>[2x]GSMAKIEKNAPTMEKKPELFNIMEVDGVPTLILSKEWWEKVCNFQAKPDDLILATYPKSGTTWMHEILDMILNDGDVEKCKRAQTLDRHAFLELKF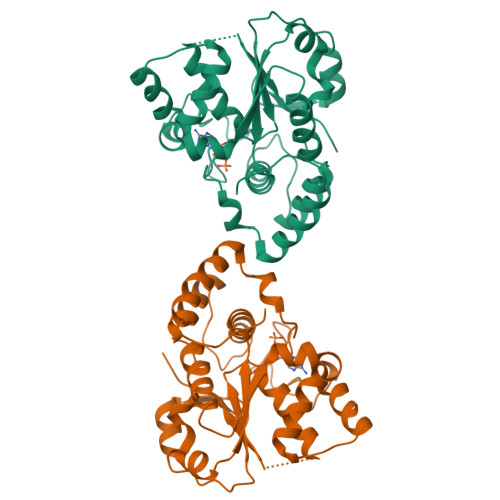PHKEKPDLEFVLEMSSPQLIKTHLPSHLIPPSIWKENCKIVYVARNPKDCLVSYYHFHRMASFMPDPQNLEEFYEKFMSGKVVGGSWFDHVKGWWAAKDMHRILYLFYEDIKKDPKREIEKILKFLEKDISEEILNKIIYHTSFDVMKQNPMTNYTTLPTSIMDHSISPFMRKGMPGDWKNYFTVAQNEEFDKDYQKKMAGSTLTFRTEI> IESIIKTATDTVKSEINAELGVVPSLNAVETGASSNTEPEEAIQTRTVINQHGVSETLVENFLSRAALVSKRSFEYKNHTSSEARTDKNFYKWTINTKSFVQLRRKLELFTYLRFDAEITILTTVAVGSNNSTYMGLPDLTLQAMFVPTGALTPEKQDSFHWQSGSNASVFFKVSDPPARMTIPFMCINSAYSVFYDGFAGFEKNGLYGINPADTIGNLCVRIVNEHQPIGFTVTVRVYMKPKHIKAWAPRPPRTLP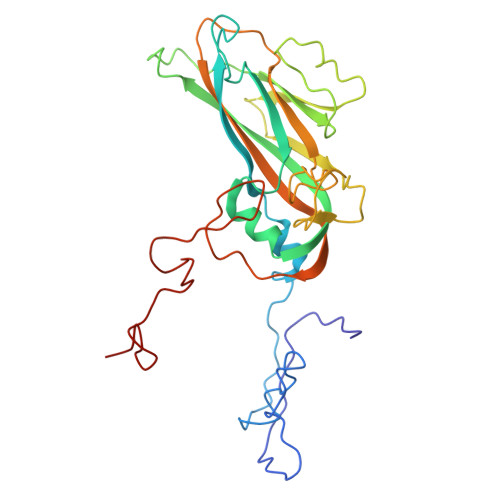YMSIANANYKGKERAPNALNAIIGNRESVKTMPHDIVLV>[4x]VDSVYRTRSLGVAAEGIPDQYADGEAARVWQLYIGDTRSRTAEYKAWLLGLLRQHGCHRVLDVACGTGVDSIML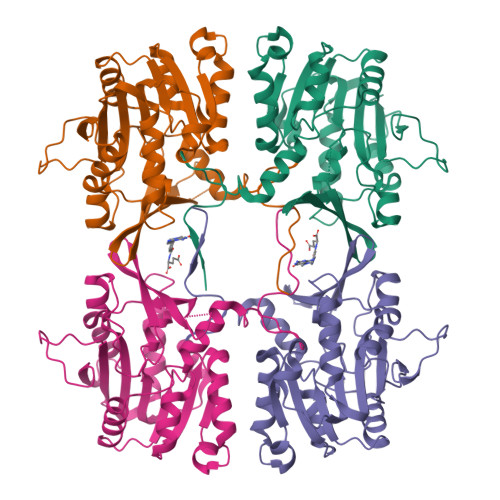VEEGFSVTSVDASDKMLKYALKERWNRRKEPAFDKWVIEEANWLTLDKDVPAGDGFDAVICLGNSFAHLPDSKGDQSEHRLALKNIASMVRPGGLLVIDHRNYDYILSTGCAPPGKNIYYKSDLTKDITTSVLTVNNKAHMVTLDYTVQVPGAGRDGAPGFSKFRLSYYPHCLASFTELVQEAFGGRCQHSVLGDFKPYRPGQAYVPCYFIHVLKKTG Insect Toll receptors perform critical functions in both embryogenesis and innate immunity. Toll receptors are activated by a complementary family of six cytokine-like molecules called Spaetzle (Spz). Three oligomeric states of the receptor were observed at near-atomic resolutions, suggesting that Toll5A is highly dynamic in the presence of Spz1C.

By contrast unbound receptors form head-to-head homodimers that keep the juxtamembrane regions far apart in an inactive conformation. The structure of Toll5A homodimers (chains A and B) was solved at the highest overall resolutions (3.4–4.4 Å), with a head-to-head arrangement, maintaining the C-terminal juxtamembrane regions far apart. The Cα atoms of Cys-783 at the C-termini of each receptor chain are separated by 207 Å. Such a structural arrangement –if sterically possible when the receptor is expressed on the same cell– would ensure that Toll5A is locked in an inactivate state preventing TIR domain association and signalling. If receptors are situated on neighbouring cells, such an orientation might be relevant to cell adhesion. The buried surface area is about 1000 Å2. Interestingly, receptor-receptor contacts in Toll5A differ from those observed in Drosophila Toll structures, which involve the N-terminal capping region and the hinge region between LRR domains. The Toll5A homodimer interface overlaps with the Spz1C ligand binding site, which suggests a direct competition between receptor-receptor and receptor-ligand interactions. Moreover, the presence of unliganded receptor in the Toll5A-Spz1C sample suggests that ligand binding is reversible.

>[2x]TSTKRFTCPEESEASNCSCEEFPSKTHFYCPDFNPTLYVDVEDRMRVDFKCYDEPHDFKSLPNLAIGSVKLLTVVDCVLDDDRPILESFKFLEVADVRSFVYNNHENGIRYNAKYFEGMEQLENLTLARGVVSIDRDTFSGFLNLKRLTIEHNKLNLQPGTFEALSNLTYLGLVYNGLNEIQPGLFDGLESLEALSLSYNDIKSLSAGSFNGLSSLRMLNLRVNKIESFDANTFASLKELSRLEITLNPFVSLPRGLFSENKKLKTLILTNNRKLVTLPEELLANLKELTVVNLSHNGVGNLPESLLSGSSGIIELNLGYNRLNSLPEELLSDQPQLQVLNLDHNQLESIPDYFLERNVELQTLYLSHNRLRSLSEKAFTKLKNLKELHLENNQLQTIPQFLFSGTPKLEEIYMQNNQLALHANSFINEELSIADNDNTPFQVLQKLRILHLRNNSISTIFQDWYINNLEMQSLDLSFNKLPGLSYTQLQFQSNITLNLSNNEISQVLLIDDLDLQPYQRINVDLNHNPLNCNCNALKFIQLIQSKAEHGLQFNVDQLRCSEPPNLLDATMDQLQTKDLLCDFESADDCPKDCQCAMRLLDHTVIVNCSGRGLTEFPDLPIPSQLHEDFNALEVHVENNRLTKLPNLTKHNEITQLYARNNSIQNLLPHNIPSKLRIIDLSQNLLKMIDDSTLAQINRSSHLETIRLSQNQWLCDCPASSFLIFVQQNSRLISDMSAIRCHPSGKSLDSITVNELCFEDYTTENLYFQ5-ethyl-4-fluoro-2-(2-nitrophenoxy)phenol | C14 H12 F N O4 | 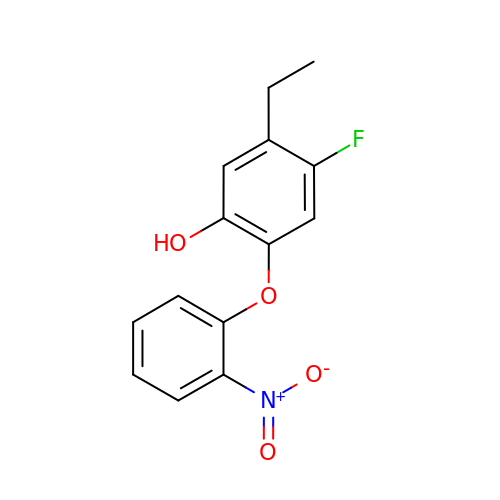XQDRDJODNDLLTL-UHFFFAOYSA-N>[4x]MAHHHHHHVDDDDKENLYFQSKPNLSAKDLALLLFTHLPGNNTPFHILAQVLSKIAYKSGKSGAFLDAFHQILSEGENAQAALTRLSRTFDAFLGVVPPVI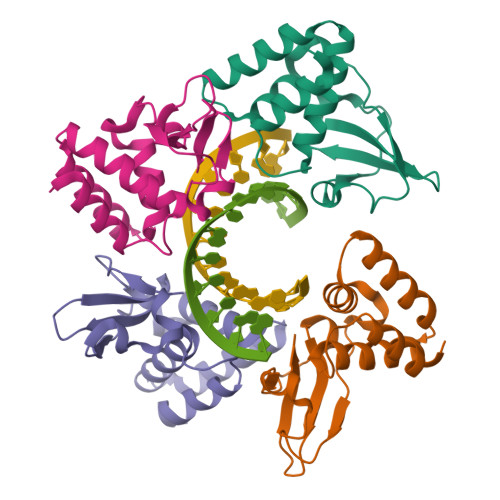RVKNFQTVPRPCQKSLRAVPPNPTIDKGWVCVYSSEQGETRALKI>[2x]GHMTPGMKIFIDPFTFEDPNEAVREFAKEIDISCVKIEQVIGAGEFGEVCSGHLKLPGKREIFVAIKTLKSGYTEKQRRDFLSEASIMGQFDHPNVIHLEGVVTKSTPVMIITEFMENGSLDSFLRQNDGQFTVIQLVGMLRGIAAGMKYLADMNYVHRDLAARNILVNSNLVCKVSDFGLSRFLEDDTSDPTYTSALGGKIPIRWTAPEAIQYRKFTSASDVWSYGIVMWEVMSYGERPYWDMTNQ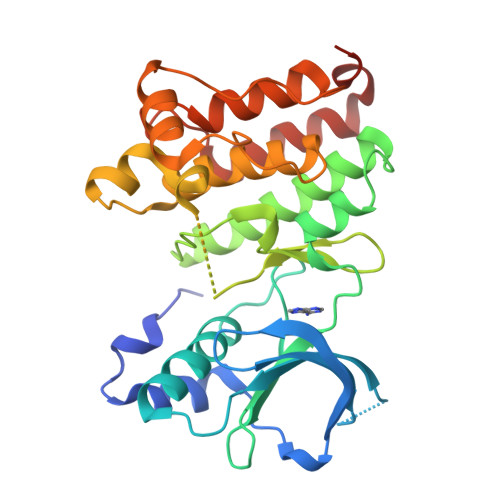DVINAIEQDYRLPPPMDCPSALHQLMLDCWQKDRNHRPKFGQIVNTLDKMIRNPNSLKAMAPLSS>GSHMRRLQQTQAQVDEVVDIMRVNVDKVLERDQKLSELDDRADALQAGASQFETSAAKLKRKYWWKNLKMMIILGVICAIILIIIIVYFST[2x];>[2x]GSHMDSSISKQALSEIETRHSEIIKLENSIRELHDMFMDMAMLVESQGEMIDRI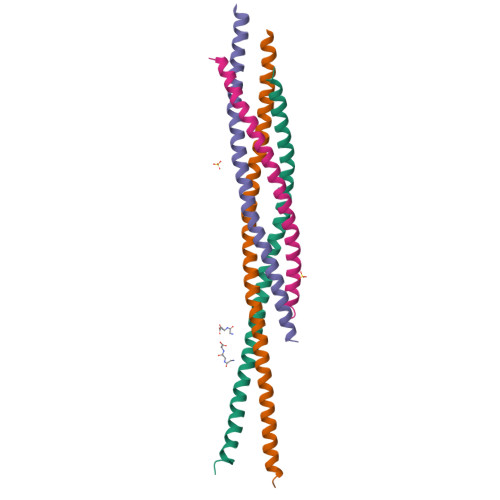EYNVEHAVDYVERAVSDTKKAVKYQSKARRKKIMIIICCVILGIIIASTIGGIFG;>GSHMRNELEEMQRRADQLADESLESTRRMLQLVEESKDAGIRTLVMLDEQGEQLDRVEEGMNHINQDMKEAEKNLKDLGK[2x];>GSHMARENEMDENLEQVSGIIGNLRHMALDMGNEIDTQNRQIDRIMEKADSNKTRIDEANQRATKMLG[2x]>[2x]MLAKDKVALLIGNMNYREHPKLKAPLVDVYELTNLLRQLDFKVVSLLDL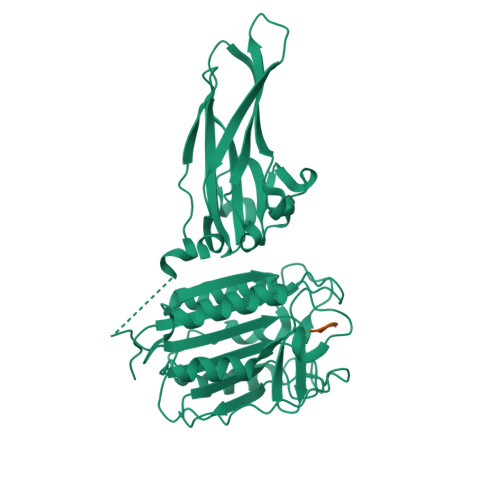TEYEMRNAVDEFLLLLDKGVYGLLYYAGHGYENFGNSFMVPVDAPNPYRSENCLCVQNILKLMQEKETGLNVFLLDMCRKRNDYDDTIPILDALKVTANIVFGYATCQGAEAFEIQHSGLANGIFMKFLKDRLLEDKKITVLLDEVAEDMGKCHLTKGKQALEIRSSLSEKRALTDPIQGTEYSAESLVRNLQWAKAHELPESMCLKFDCGVQIQLGFAAEFSNVMIIYTSIVYKPPEIIMCDAYVTDFPLDLDIDPKDANKGTPEETGSYLVSKDLPKHCLYTRLSSLQKLKEHLVFTVCLSYQYSGLEDTVEDKQEVNVGKPLIAKLDMHRLEHHHHHH> MASHHHHHHSGMTWLEPQIKSQLQSERKDWEANEVGAFLKKAPERKEQFHTIGDFPVQRTYTAADIADTPLEDIGLPGRYPFTRGPYPTMYRSRTWTMRQIAGFGTGEDTNKRFKYLIAQGQTGISTDFDMPTLMGYDSDHPMSDGEVGREGVAIDTLADMEALLADIDLEKISVSFTINPSAWILLAMYVALGEKRGYDLNKLSGTVQADILKEYMAQKEYIYPIAPSVRIVRDIITYSAKNLKRYNPINISGYHISEAGSSPLQEAAFTLANLITYVNEVTKTGMHVDEFAPRLAFFFVSQGDFFEEVAKFRALRRCYAKIMKERFGARNPESMRLRFHCQTAAATLTKPQYMVNVVRTSLQALSAVLGGAQSLHTNGYDEAFAIPTEDAMKMALRTQQIIAEESGVADVIDPLGGSYYVEALTTEYEKKIFEILEEVEKRGGTIKLIEQGWFQKQIADFAYETALRKQSGQKPVIGVNRFVENEEDVKIEIHPYDNTTAERQISRTRRVRAERDEAKVQAMLDQLVAVAKDESQNLMPLTIELVKAGATMGDIVEKLKGI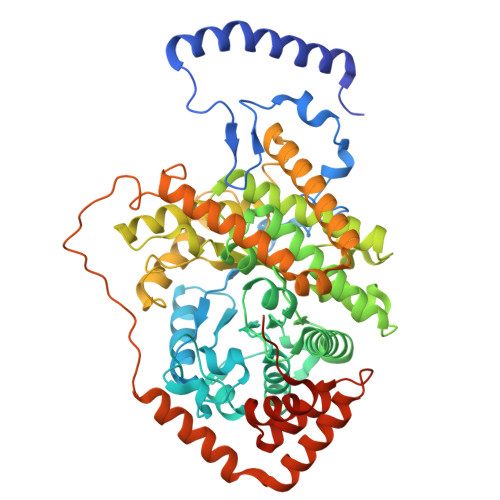WGTYRETPVFGSAWSHPQFEK>ADQPIDADVTVIGSGPGGYVAAIKAAQLGFKTVCIEKNETLGGTCLNVGCIPSKALLNNSHYYHMAHGKDFASRGIEMSEVRLNLDKMMEQKSTAVKALTGGIAHLFKQNKVVHVNGYGKITGKNQVTATKADGGTQVIDTKNILIATGSEVTPFPGITIDEDTIVSSTGALSLKKVPEKMVVIGAGVIGVELGSVWQRLGADVTAVEFLGHVGGVGIDMEISKNFQRILQKQGFKFKLNTKVTGATKKSDGKIDVSIEAASGGKAEVITCDVLLVCIGRRPFTKNLGLEELGIELDPRGRIPVNTRFQTKIPNIYAIGDVVAGPMLAHKAEDEGIICVEGMAGGAVHIDYNCVPSVIYTHPEVAWVGKSEEQLKEEGIEYK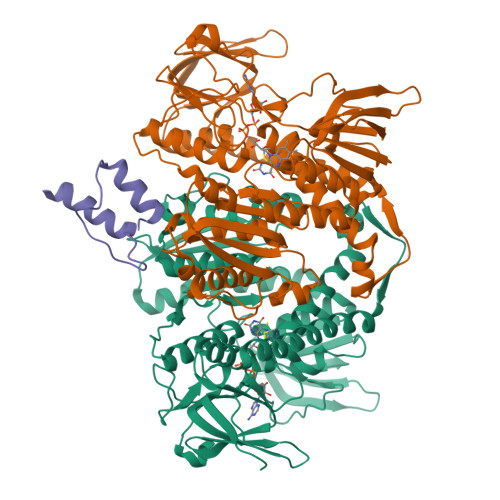VGKFPFAANSRAKTNADTDGMVKILGQKSTDRVLGAHILGPGAGEMVNEAALALEYGASCEDIARVCHAHPTLSEAFREANLAASFGKSINF[10x];>GDPIKILMPSLSPTMEEGNIVKWLKKEGEAVSAGDALCEIETDKAVVTLDASDDGILAKIVVEEGSKNIRLGSLIGLIVEEGEDWKHVEIPKDVGPPPPVSKPSEPRPSPEPQISIPVKKEHIPGTLRFRLSPAARNILEKHSLDASQGTATGPRGIFTKEDALKLVQLKQTGKITESRPTPAPTATPTAPSPLQATSGPSYPRPVIPPVSTPGQPNAVGTLEHHHHHH[5x]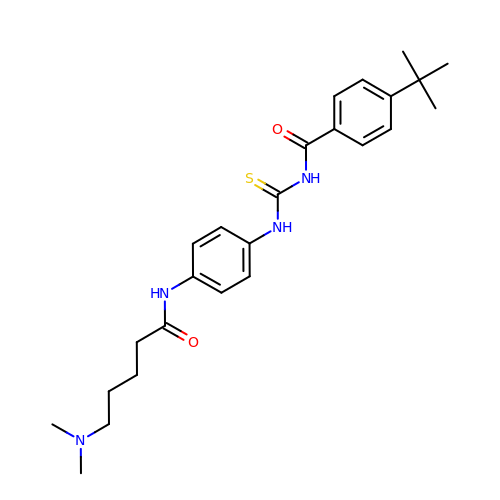4-~{tert}-butyl-~{N}-[[4-[5-(dimethylamino)pentanoylamino]phenyl]carbamothioyl]benzamide | C25 H34 N4 O2 S | BVJSXSQRIUSRCO-UHFFFAOYSA-N>MTVVPITSPDLDAAE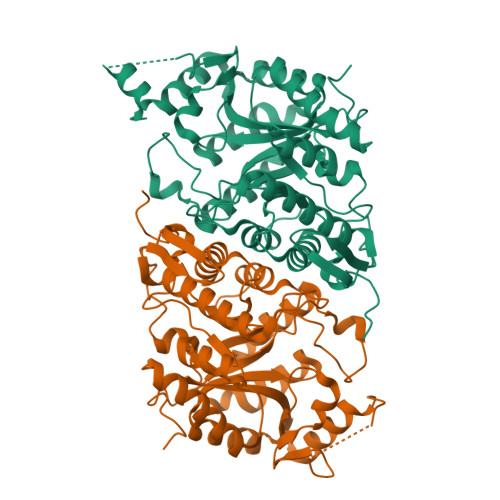VSWFAALCSDDYAYLGVPDDALKSSFEHCSEIVTRAETLGFRNILCPSSYQVGQDTLSFVAACSQITERINLLAAIRCGEMQPIMLARTVATLDHMLKGRLTLNVISSDFPGEVADSAFRYRRSHEVVQILRQAWTRDTIDHEGEVYNFKGVTTEPARPYQQNGGPLLYFGGYSPDALELCGAQCDVYLMWPEPKEQIAERMKAVHARAEAHGRTLDYGLRVHMIVRDTEKEARDYAEHLVSKLDDEYGRLIRSRAHDSTSLGVSHQARTRELADKFGYVERHLWTGIGRARSGCGAALVGSTDQVLSEIEAYKKMGVRAFIFSGYPHLDEAEHFGKKVLPQLKTCSLPHIYGRVPADTPATPLGAGRRHLEHHHHHH[2x]> IVGGYTCGANTVPYQVSLNSGYHFCGGSLINSQWVVSAAHCYKSGIQVRLGEDNINVVEGNEQFISASKSIVHPSYNSETYNNDIMLIKLKSAASLNSRVASISLPTSCASAGTQCLISGWGNTKSSGTSYPDVLKCLKAPILSDSSCKSASSFIITSNMFCAGYLEGGKDACQGDSGGPVVCSGKLQGIVSWGSGCAQKNKPGIYTKVCNYVSWIKQTI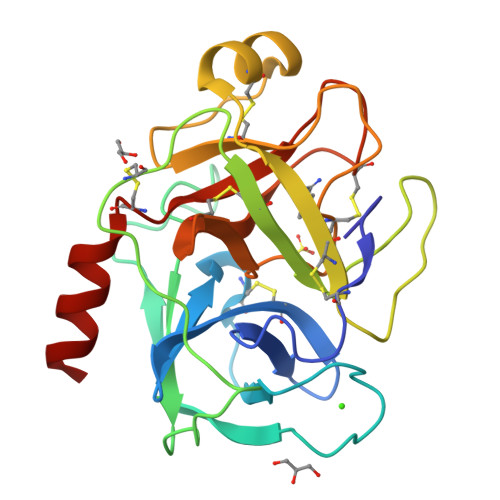ASN>MGHHHHHHAENLYFQGHMLRLSAPGQLDDDLCLLGDVQVPVFLLRLGEASWALVEGGISR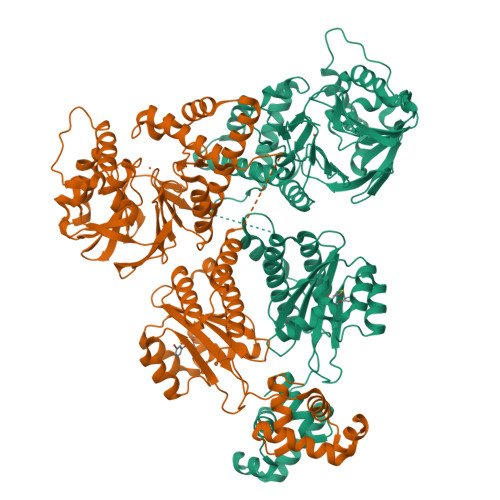DAELVWADLCRWVADPSQVHYWLITHKHYDHCGLLPYLCPRLPNVQVLASERTCQAWKSESAVRVVERLNRQLLRAEQRLPEACAWDALPVRAVADGEWLELGPRHRLQVIEAHGHSDDHVVFYDVRRRRLFCGDALGEFDEAEGVWRPLVFDDMEAYLESLERLQRLPTLLQLIPGHGGLLRGRLAADGAESAYTECLRLCRRLLWRQSMGESLDELSEELHRAWGGQSVDFLPGELHLGSMRRMLEILSRQALPLDSGSETPGTSESATPESGPGTMRNDGGFLLWWDGLRSEMQPIHDSQGVFAVLEKEVRRLGFDYYAYGVRHTIPFTRPKTEVHGTYPKAWLERYQMQNYGAVDPAILNGLRSSEMVVWSDSLFDQSRMLWNEARDWGLCVGATLPIRAPNNLLSVLSVARDQQNISSFEREEIRLRLRCMIELLTQKLTDLEHPMLMSNPVCLSHREREILQWTADGKSSGEIAIILSISESTVNFHHKNIQKKFDAPNKTLAAAYAAALGLI[2x]> XSLSAAEADLAGKSWAPVFANKNANGLDFLVALFEKFPDSANFFADFKGKSVADIKASPKLRDVSSRIFTRLNEFVNNAANAGKMSAMLSQFAKEHVGFGVGSAQFENVRSMFPGFVASVAAPPAGADAAW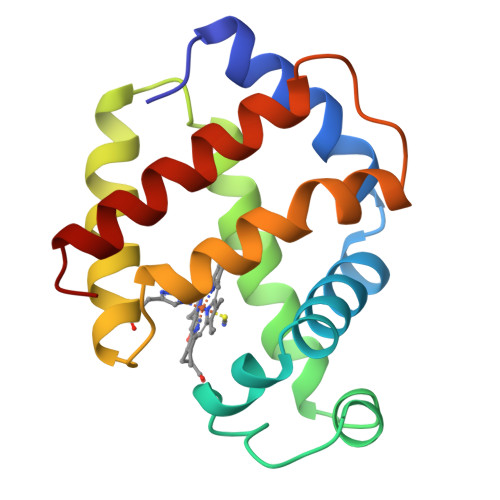TKLFGLIIDALKAAGK>MTADELVFFVNGKKVVEKNADPETTLLVYLRRKLGLCGTKLGCGEGGCGACTVMISKYDRLQNKIVHFSVNACLAPICSLHHVAVTTVEGIGNTQKLHPVQERIARSHGSQCGFCTPGIVMSMYTLLRNQPEPTVEEIENAFQGNLCRCTGYRPILQGFRTFAKDGGCCGGSGNNPNCCMNQTKDQTVSLSPSLFNPEDFKPLDPTQEPIFPPELLRLKDTPQKKLRFEGERVTWIQASTMEELLDLKAQHPDAKLVVGNTEIGIEMKFKNMLFPLIVCPAWIPELNSVVHGPEGISFGASCPLSLVESVLAEEIAKLPEQKTEVFRGVMEQLRWFAGKQVKSVASIGGNIITASPISDLNPVFMASGAKLTLVSRGTRRTVRMDHTFFPGYRKTLLRPEEILLSIEIPYSKEGEFFSAFKQASRREADIAKVTSGMRVLFKPGTIEVQELSLCFGGMADRTISALKTTPKQLSKSWNEELLQSVCAGLAEELQLAPDAPGGMVEFRRTLTLSFFFKFYLTVLQKLGRADLEDMCGKLDPTFASATLLFQKDPPANVQLFQEVPKDQSEEDMVGRPLPHLAANMQASGEAVYCD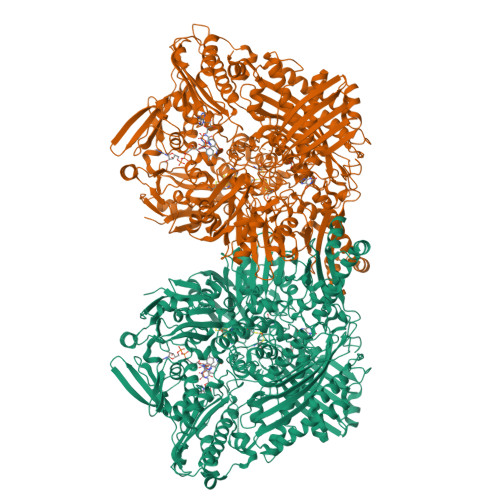DIPRYENELSLRLVTSTRAHAKITSIDTSEAKKVPGFVCFLTAEDVPNSNATGLFNDETVFAKDEVTCVGHIIGAVVADTPEHAQRAARGVKITYEDLPAIITIQDAINNNSFYGSEIKIEKGDLKKGFSEADNVVSGELYIGGQEHFYLETNCTIAVPKGEAGEMELFVSTQNTMKTQSFVAKMLGVPDNRIVVRVKRMGGGFGGKETRSTVVSTALALAAHKTGRPVRCMLDRDEDMLITGGRHPFLAKYKVGFMKTGTVVALEVAHFSNGGNTEDLSRSIMERALFHMDNAYKIPNIRGTGRICKTNLPSNTAFRGFGGPQGMLIAEYWMSEVAITCGLPAEEVRRKNMYKEGDLTHFNQKLEGFTLPRCWDECIASSQYLARKREVEKFNRENCWKKRGLCIIPTKFGISFTLPFLNQGGALVHVYTDGSVLLTHGGTEMGQGLHTKMVQVASRALKIPTSKIHISETSTNTVPNTSPTAASASADLNGQGVYEACQTILKRLEPFKKKKPTGPWEAWVMDAYTSAVSLSATGFYKTPNLGYSFETNSGNPFHYFSYGVACSEVEIDCLTGDHKNLRTDIVMDVGSSLNPAIDIGQVEGAFVQGLGLFTMEELHYSPEGSLHTRGPSTYKIPAFGSIPIEFRVSLLRDCPNKRAIYASKAVGEPPLFLASSIFFAIKDAIRAARAQHGDNAKQLFQLDSPATPEKIRNACVDQFTTLCVTGVPENCKSWSVRI[2x]> MTRDEMISVEPEAAELQDQHRRDFLKRSGAAVLSLSLSSLATGVVPGFLKDAQAGTKAPGYASWEDIYRKEWKWDKVNWGSHLNICWPQGSCKFYVYVRNGIVWREEQAAQTPACNVDYVDYNPLGCQKGSAFNNNLYGDERVKYPLKRVGKRGEGKWKRVSWDEAAGDIADSIIDSFEAQGSDGFILDAPHVHAGSIAWGAGFRMTYLMDGVSPDINVDIGDTYMGAFHTFGKMHMGYSADNLLDAELIFMTCSNWSYTYPSSYHFLSEARYKGAEVVVIAPDFNPTTPAADLHVPVRVGSDAAFWLGLSQVMIDEKLFDRQFVCEQTDLPLLVRMDTGKFLSAEDVDGGEAKQFYFFDEKAGSVRKASRGTLKLDFMPALEGTFSARLKNGKTIQVRTVFEGLREHLKDYTPEKASAKCGVPVSLIRELGRKVAKKRTCSYIGFSSAKSYHGDLMERSLFLAMALSGNWGKPGTGAFAWAYSDDNMVYLGVMSKPTAQGGMDELHQMAEGFNKRTLEADPTSTDEMGNIEFMKVVTSAVGLVPPAMWLYYHVGYDQLWNNKAWTDPALKKSFGAYLDEAKEKGWWTNDHIRPAPDKTPQVYMLLSQNPMRRKRSGAKMFPDVLFPKLKMIFALETRMSSSAMYADIVLPCAWYYEKHEMTTPCSGNPFFTFVDRSVAPPGECREEWDAIALILKKVGERAAARGLTEFNDHNGRKRRYDELYKKFTMDGHLLTNEDCLKEMVDINRAVGVFAKDYTYEKFKKEGQTRFLSMGTGVSRYAHANEVDVTKPIYPMRWHFDDKKVFPTHTRRAQFYLDHDWYLEAGESLPTHKDTPMVGGDHPFKITGGHPRVSIHSTHLTNSHLSRLHRGQPVVHMNSKDAAELGIKDGDMAKLFNDFADCEIMVRTAPNVQPKQCIVYFWDAHQYKGWKPYDILLIGMPKPLHLAGGYEQFRYYFMNGSPAPVTDRGVRVSIKKA;> MTYVQDGNKSELRKAKRQLVTVIDLNKCLGCQTCTVACKNIWTKRPGTEHMRWNNVTTYPGKGYPRDYERKGGGFLRGEPQPGVLPTLIDSGDDFQFNHKEVFYEGKGQTVHFHPTSKSTGKDPAWGYNWDEDQGGGKWPNPFFFYLARMCNHCTNPACLAACPTGAIYKREDNGIVLVDQERCKGHRHCVEACPYKAIYFNPVSQTSEKCILCYPRIEKGIANACNRQCPGRVRAFGYLDDTTSHVHKLVKKWKVALPLHAEYGTGPNIYYVPPMGARGFGEDGEITDKTRIPLDVLEGLFGPEVKRVLAVLHTERENMRAGRGSELMDLLISKKWSDRFGGFTNDPLTQS;> MKAKRVPGGKELLLDLDAPIWAGAESTTFEMFPTPLVMVKEVSPFLALSEGHGVIKRLDVAALHNGSMIA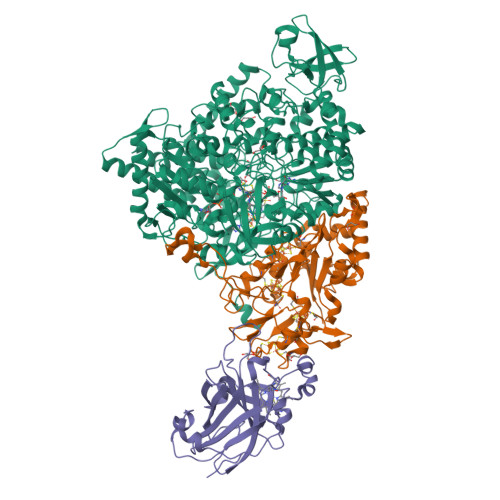LRLKWASEKHDKIVDLNSFVDGVGAMFPVARGAQAVTMGATGRPVNAWYWKANANEPMEIVAEGFSAVRRMKDKAGSDLKAVAQHRNGEWNVILCRSMATGDGLAKLQAGGSSKIAFAVWSGGNAERSGRKSYSGEFVDFEILK>MDDNVNDFRPVPYPDEVVGLNPDPDFEPIWEIASPTITVFSSKASNDISYRVPAIAVTKKGSILVFCEARYGTWQDKAGRTDILMKRSTDKGITWTEKNLTNQATSSKLSYMDPTVVVDQVTGKIFLFTSLWDAVGKESAKQGYNNRAIMYTSEDDGLNWTRKDLTDEVEIGIFSGATRMIGSFGPGSGVQMTSSEQYKNRLIVPIRTFKVNEAAGTVSNGGNTAMWSDDNGGTWETGQPNKSGEWMVTEAPDGALIGNIRYNGHRQNYVSTDGGAKWPSFSDYDPIALPTPAKGCAGSVIVKDGWMYYCGAKGIIETTAHDDRGILYLAKAKFFGGHSHTFDPADHMVLYDKAAGYT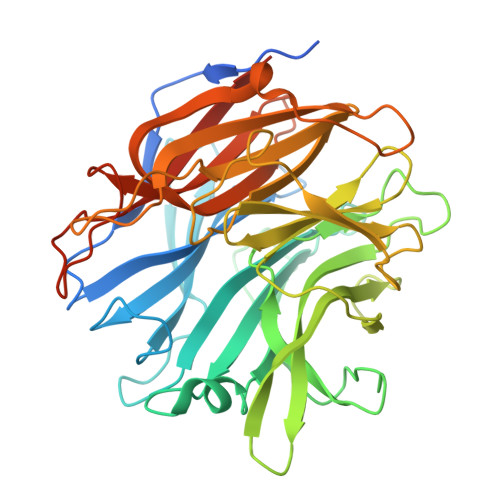CMALLPDGDMAIVAELGNEPGFQKLSTRPAEWMRLELFILSTKKPLHHHHHHHHHH[2x]>[6x]SNAKSVIE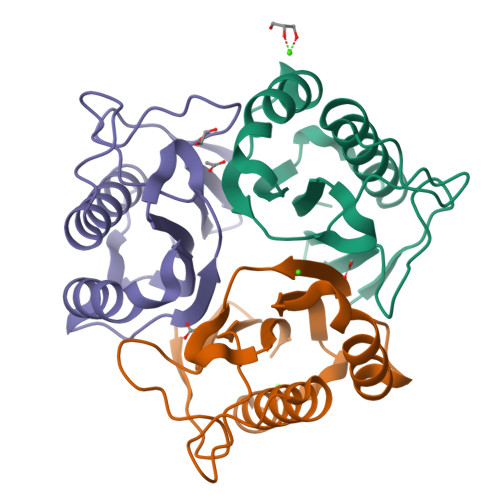TKNAPSAIGPYSQAICFNGILYASGQIPINPDTGDLVENDIEKQTRQVLKNIDAVLLQAGTTKDKIVKTTIFITNINNSSQVNDIYADYFKGTIFPARSTVEVSALPKGALVEIEVIAGV Abscisic acid (ABA) is a phytohormone essential to the regulation of numerous aspects of plant growth and development. ABCG25 in Arabidopsis thaliana has been identified to be an ABA exporter and play roles in regulating stomatal closure and seed germination. As a ‘half-transporter’ with only one NBD and one transmembrane domain (TMD) in a polypeptide chain, ABCG25 forms a homodimer as a functional unit, similar to other determined ‘half-transporter’ ABCG structures including the human cholesterol transporter ABCG1 (hABCG1) and multidrug transporter ABCG2 (hABCG2)39–47. In this study, we determined the high-resolution structures of ABCG25 in Arabidopsis thaliana in the apo, ABA-bound and ATP-bound states using cryogenic electron microscopy (cryo-EM) single particle analysis.

We generated a catalytic mutant by replacing the glutamate residue E232 in the conserved Walker B motif of the nucleotide-binding domain (NBD) with a glutamine (named ABCG25EQ hereafter). The ABCG25EQ mutant had an almost abolished ATP hydrolysis activity, which is suitable to trap ABCG25 in the ATP-bound state. We purified this mutant and incubated it with ATP and Mg2+ before cryo-sample preparation. An EM map with an overall resolution of 3.0 Å was finally obtained. Clear densities were observed in each NBD, fitting well with the ATP molecule and Mg2+. ATP forms intense interactions with residues from both NBDs, thus pulling NBDs close together. A section view of the electrostatic potential surface reveals that the intracellular cavity observed in the apo or ABA-bound state disappears and the transmembrane region of ABCG25 is sealed to both sides of the membrane. ATP binding leads to closure of the NBDs and such large movements are transduced to the TMDs through the three-helix bundle formed by CnH, CpH of the TMD and E-helix of the NBD. The extracellular gate remains closed at this state, with Y564 and Y565 forming the plugging residues. Thus, the ATP-bound structure of ABCG25EQ may represent a state during the transport cycle when the bound ABA is released from the intracellular cavity when the extracellular gate is transiently open, and the extracellular gate closes again, ready to reset to the resting state after ATP hydrolysis and ADP release.

>[2x]MSAFDGVENQMNGPDSSPRLSQDPREPRSLLSSSCFPITLKFVDVCYRVKIHGMSNDSCNIKKLLGLKQKPSDETRSTEERTILSGVTGMISPGEFMAVLGPSGSGKSTLLNAVAGRLHGSNLTGKILINDGKITKQTLKRTGFVAQDDLLYPHLTVRETLVFVALLRLPRSLTRDVKLRAAESVISELGLTKCENTVVGNTFIRGISGGERKRVSIAHELLINPSLLVLDQPTSGLDATAALRLVQTLAGLAHGKGKTVVTSIHQPSSRVFQMFDTVLLLSEGKCLFVGKGRDAMAYFESVGFSPAFPMNPADFLLDLANGVCQTDGVTEREKPNVRQTLVTAYDTLLAPQVKTCIEVSHFPQDNARFVKTRVNGGGITTCIATWFSQLCILLHRLLKERRHESFDLLRIFQVVAASILCGLMWWHSDYRDVHDRLGLLFFISIFWGVLPSFNAVFTFPQERAIFTRERASGMYTLSSYFMAHVLGSLSMELVLPASFLTFTYWMVYLRPGIVPFLLTLSVLLLYVLASQGLGLALGAAIMDAKKASTIVTVTMLAFVLTGGYYVNKVPSGMVWMKYVSTTFYCYRLLVAIQYGSGEEILRMLGCDSKGKQGASAATSAGCRFVEEEVIGDVGMWTSVGVLFLMFFGYRVLAYLALRRIKH> MEEVKKKLEEVWKKAKEDAGDNEKFLELLELILENPEILEILELYVFINKEDVVEKLFDVIKKAVEDAGDNEKFLELLKEMLSNPEIFEILLEYVYIKKEDVVEKLFEVIKQAVEDAGDNPVFLKLLKKMISNPEIFEILLEYVYIGKEEVVKKFFEVIKQAVEDAGNNPIFLKLLEKIILDPERFKKLLEKVEVGEEEEVKAEFKEIKKAVEEAGNDPIKLKELEEKLGSWLEHHHHHH

Here we describe a systematic approach to generating modular and rigid repeat protein oligomers with coincident C2 to C8 and superhelical symmetry axes that can be readily extended by repeat propagation. Repeat proteins are composed of an asymmetric structural motif that is concatenated several times in tandem within a single protein chain. From these building blocks, we demonstrate that a wide range of unbounded fibres can be systematically designed by introducing hydrophilic surface patches that force staggering of the monomers; the geometry of such fibres can be precisely tuned by varying the number of repeat units in the monomer and the placement of the hydrophilic patches. All multiplexes follow the naming convention CsHRN_Rr where s is the cyclic symmetry, HR stands for helical repeat, R is the number of repeats in a single chain and N is an index to differentiate between multiplexes of the same symmetry.

We determined the high-resolution structures of five designs from C2 to C6 symmetry by X-ray crystallography, cryogenic electron microscopy (cryoEM) or both. For C3HR3_4r, the overall C-alpha r.m.s.d. between the crystal structure and design model is 1.21 Å. In contrast to C2HR1_4r, C3HR3_4r has a large twist, causing the interface to become staggered, with the top two repeats packing on the bottom two repeats of the adjacent monomer. Notably, C3HR3 was verified to high resolution for the bounded four-repeat, bounded eight-repeat and unbounded fibre designs.> GPLGSSEQLKHCNGILKELLSKKHAAYAWPFYKPVDASALGLHDYHDIIKHPMDLSTVKRKMENRD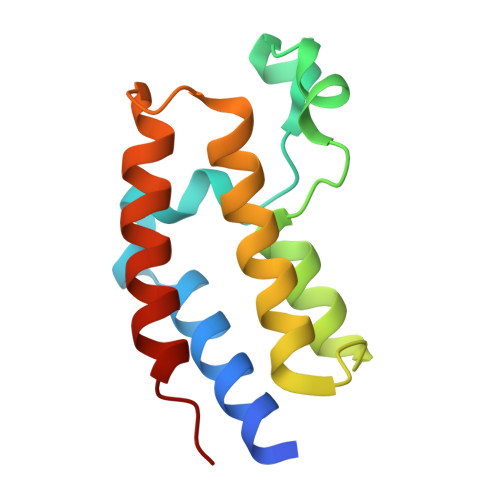YRDAQEFAADVRLMFSNCYKYNPPDHDVVAMARKLQDVFEFRYAKMPD>MEYTQLGRIGLKVSRLVLGTMNFGPTTDEAESHAIMDAALDAGINFFDTANVYGWGENKGRTEEILGSWFAQGGDRRDKVVLATKVYGNMGLDGPAWPNHDKLSALNIRRSVDASLKRLGTDHIDLYQFHHVDRDTPWDEIWQAMDVLVRQGKILYVGSSNFAGWNIAQANETAARHGRLGLVSEQCLYNLCERRAEMEVVPAAREYGLGVIAWSPLHGGLLGGAIRKEQEGGNRRAASGRAADALKDPQQREQIQRYEDLLDKHGLEPGEVALAWLLTRPGVTGPIVGPRTADQLASA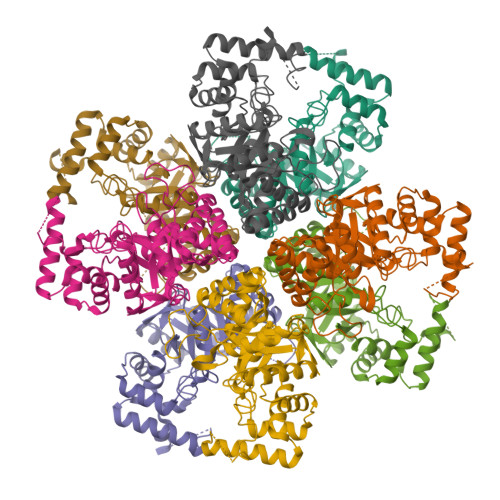VRAAELTLTDEVLTALDEIFPGPGPSPEAFAW[16x]>[2x]MKELIRKLTEAFGPSGREEEVRSIILEELEGHIDGHRIDGLGNLIVWKGSGEKKVILDAHIAEIGVVVTNVDDKGFLTIEPVGGVSPYMLLGKRIRFENGTIGVVGMEGETTEERQENVRKLSFDKLFIDIGANSREEAQK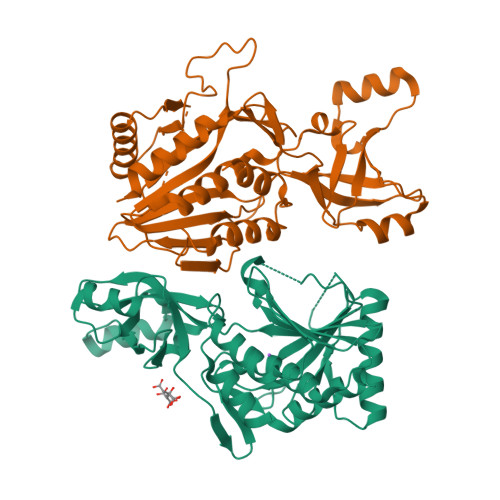MCPIGSFGVYDSGFVEVSGKYVSKAMDDRIGCAVIVEVFKRIKPAVTLYGVFSVQEEVGLVGASVAGYGVPADEAIAIDVTDSADTPKAIKRHAMRLSGGPALKVKDRASISSKRILENLIEIAEKFDIKYQMEVLTFGGTNAMGYQRTREGIPSATVSIPTRYVHSPSEMIAPDDVEATVDLLIRYLGA>FQVPMSNLLTVHQNLPALPVDATSDEVRKNLMDMFRDRQAFSEHTWKMLLSVCRSWAAWCKLNNRKWFPAEPEDVRDYLLYLQARGLAVKTIQQHLGQLNMLHRRSGLPRPSDSNAVSLVMRRIRKENVDAGERAKQALAFERTDFDQVRSLMENSDRCQDIRNL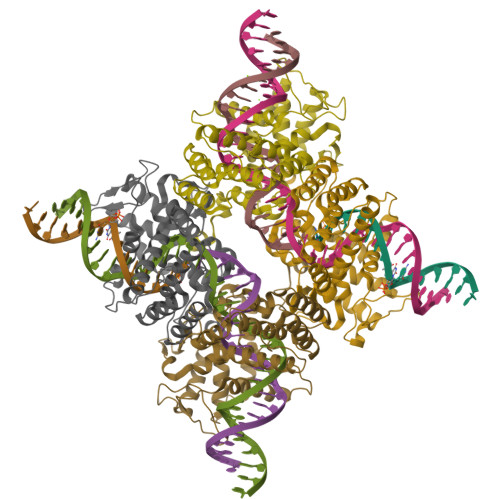AFLGIAYNTLLRIAEIARIRVKDISRTDGGRMLIHIGRTKTLVSTAGVEKALSLGVTKLVERWISVSGVADDPNNYLFCRVRKNGVAAPSATSQLSTRALEGIFEATHRLIYGAKDDSGQRYLAWSGHSARVGAARDMARAGVSIPEIMQAGGWTNVNIVMNYIRNLDSETGAMVRLLEDGD[4x]> MKELIYIEEPKILFAHGQKCTDARDGLALFGPLNNLYGIKSGVIGTKQGLKIFRDYLDHIQKPIYNSNSITRPMFPGFEAVFDCKWESTGITFKEVTNEDIGKFLYNSSTHKRTYDLVSLFIDKIISANKNEDENVDVWFVIVPDEIYKYCRPNSVLPKEMVQTKALMSKSKAKSFRY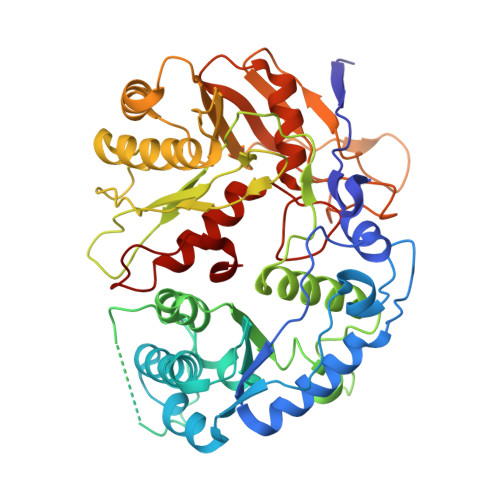EPSLFPDINIELKEQEKEAETYNYDAQFHDQFKARLLKHTIPTQIFRESTLAWRDFKNAFGLPIRDFSKIEGHLAWTISTAAFYKAGGKPWKLSDVRNGVCYLGLVYKKVEKSKNPRNACCAAQMFLDNGDGTVFKGEVGPWYNPKNGQYHLEPKEAKALLSQSLQSYKEQIGEYPKEVFIHAKTRFNHQEWDAFLEVTPKETNLVGVTISKTKPLKLYKTEGDYTILRGNAYVVNERSAFLWTVGYVPKIQTALSMEVPNPLFIEINKGEADIKQVLKDILSLTKLNYNACIFADGEPVTLRFADKIGEILTASTDIKTPPLAFKYYI N~3~-[3-(5-METHOXYPYRIDIN-3-YL)BENZYL]PYRIDINE-2,3-DIAMINE 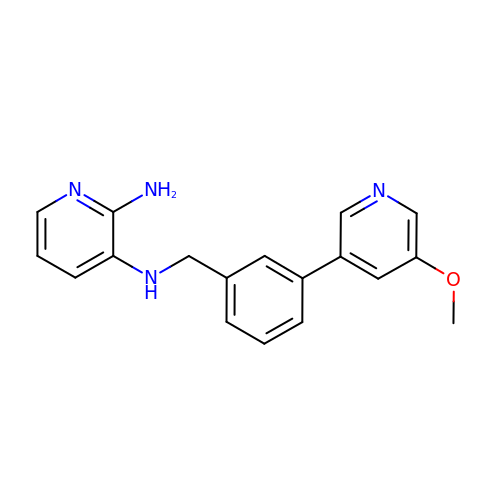| C18 H18 N4 O | PGAWZMRRCVSRIM-UHFFFAOYSA-N>[3x]MSVIEINDENFDEVIKKSDKVVVVDFWAEWCGPCRMIAPI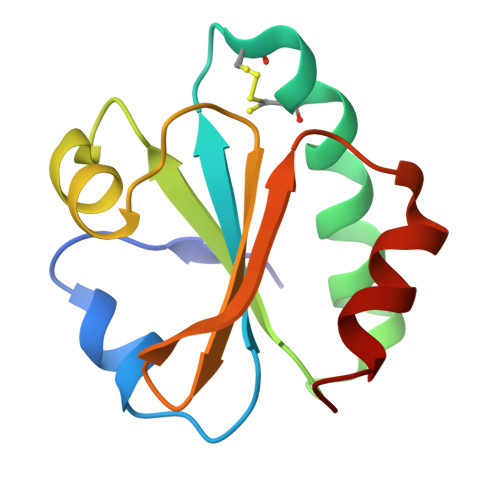IEELAEEYAGKVVFGKVNVDENPEIAAKYGIMSIPTLLFFKNGKVVDQLVGARPKEALKERIKKYL>MKINIIKAFGILLCRLKKYNPVTTGDINKFEFLFLKASYADKHWTPPKGLHENNESGLETAVRETLEETGINKDKYKLLNYQKTL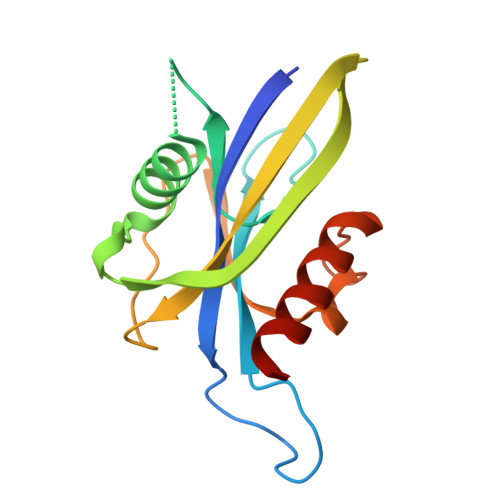KYNVKDKPKETTYYLAMLLNNEENVILSDEHTDYKWIGSHESDTYNLPESLADLLKEAEEFLNKEQL[4x]[(2R,3R,4R,6R)-3-acetamido-6-methyl-4-oxidanyl-5-oxidanylidene-oxan-2-yl] [[(2R,3S,4R,5R)-5-[2,4-bis(oxidanylidene)pyrimidin-1-yl]-3,4-bis(oxidanyl)oxolan-2-yl]methoxy-oxidanyl-phosphoryl] hydrogen phosphate | C17 H25 N3 O16 P2 | 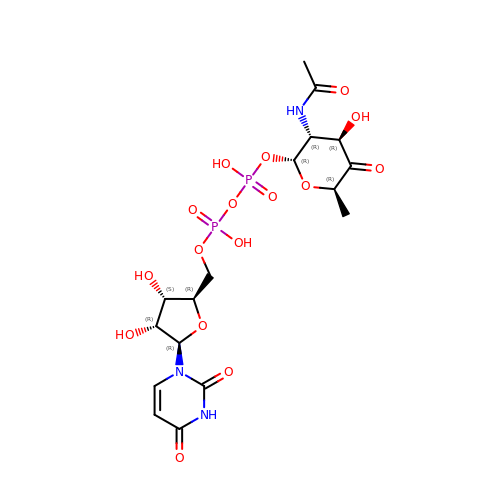XBILTLYIKDPORV-HZUXRPHDSA-N> SESKVKKVVSIPAIDEGDLWTWRKYGQKDILGSRFPRGYYRCAYKFTHGCKATKQVQRSETDSN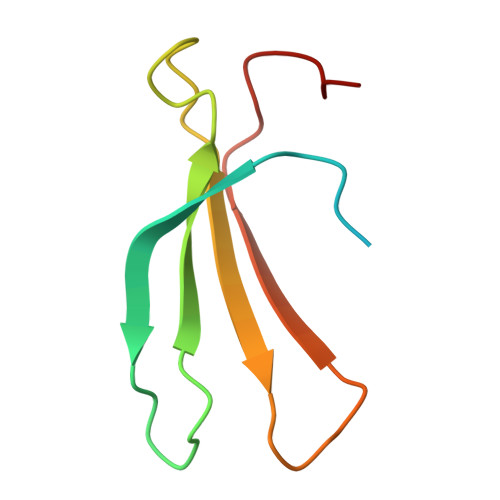MLAITYLSEHNHPRPT> LSLQPEGLRVVNLLQERNMLPSTPLKPPVPNLHEDIQKLNCNPELFRCTLTSIPQTQALLNKAKLPLGLLLHPFKDLVQLPVVTSSTIVRCRSCRTYINPFVSFLDQRRWKCNLCYRVNDVPEEFLYNPLTRVYGEPHRRPEVQNATIEFMAPSEYMLRPPQPPVYLFVFDVSHNAVETGYLNS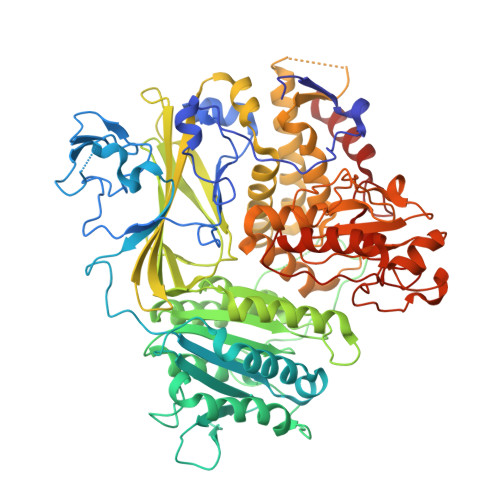VCQSLLDNLDLLPGNTRTKIGFITFDSTIHFYGLQESLSQPQMLIVSDIEDVFIPMPENLLVNLNESKELVQDLLKTLPQMFTKTLETQSALGPALQAAFKLMSPTGGRMSVFQTQLPTLGVGALKPREEPNHRSSAKDIHMTPSTDFYKKLALDCSGQQVAVDLFLLSGQYSDLASLGCISRYSAGSVYYYPSYHHQHNPVQVQKLQKELQRYLTRKIGFEAVMRIRCTKGLSIHTFHGNFFVRSTDLLSLPNVNPDAGYAVQMSVEESLTDTQLVSFQSALLYTSSKGERRIRVHTLCLPVVSTLNDVFLGADVQAISGLLANMAVDRSMTASLSDARDALVNAVIDSLSAYRSSVLSNQQPGLMVPFSLRLFPLFVLALLKQKSFQTGTNARLDERIFAMCQVKNQPLVYLMLTTHPSLYRVDNLSDEGALNISDRTIPQPPILQLSVEKLSRDGAFLMDAGSVLMLWVGKNCTQNFLSQVLGVQNYASIPQPMTDLPELDTPESARIIAFISWLREQRPFFPILYVIRDESPMKANFLQNMIEDRTESALSYYEFLLHIQQQVNK> GAMALSYSSPLRFFRNFRFHPEFTRLVAGGWRSLTYSSRIDPDKEMCPYELEGTQCPSGCSFQHFVDIT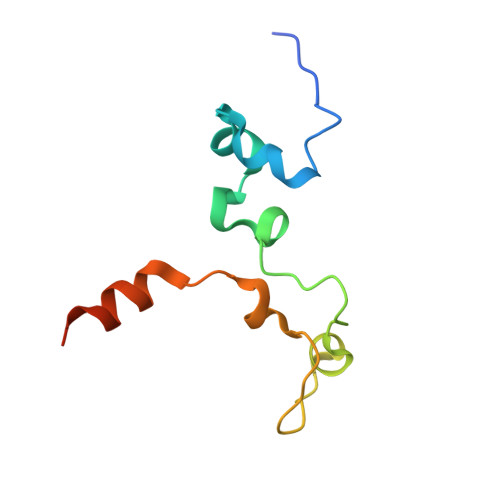PAADERILLELSGSHHHHHH>[4x]MFIEAIVLGLTALILYSVYSVKSFNTTRPTLPPVYPVTVPFLGHIVQFGKNPLEFMQRCKRDLKSGVFTISIGGQRVTIVGDPHEHSRFFSPRNEILSPREVYTFMTPVFGEGVAYAAPYPRMREQLNFLAEELTIAKFQNFVPAIQHEVRKFMAENWKEDEGVINLLEDCGAMIINTACQCLFGEDLRKRLNARHFAQLLSKMESSLIPAAVFMPWLL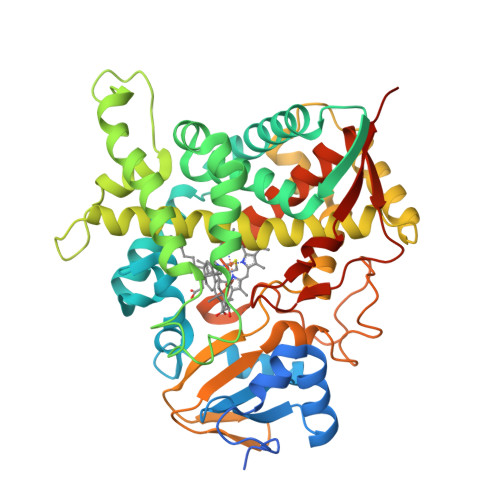RLPLPQSARCREARAELQKILGEIIVAREKEEASKDNNTSDLLGGLLKAVYRDGTRMSLHEVCGMIVAAMFAGQHTSTITTSWSMLHLMHPKNKKWLDKLHKEIDEFPAQLNYDNVMDEMPFAERCVRESIRRDPPLLMVMRMVKAEVKVGSYVVPKGDIIACSPLLSHHDEEAFPNPRLWDPERDEKVDGAFIGFGAGVHKCIGQKFALLQVKTILATAFREYDFQLLRDEVPDPDYHTMVVGPTLNQCLVKYTRKKKLPSHHHH> SNAEEELPFKVLGDGSYLFEGKTSLSDVRHYLDLPENAFGELGDEVDTLSGLFLEIKQELPHVGDTAVY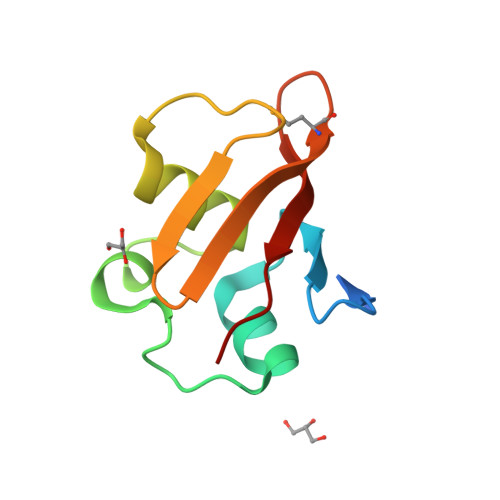EPFRFQVTQMDKRRIIEIKIFPFE>[3x]MSLNVQTVAVIGSGTMGAGIAEVAASHGHQVLLYDISAEALTRAIDGIHARLNSRVTRGKLTAETCERTLKRLI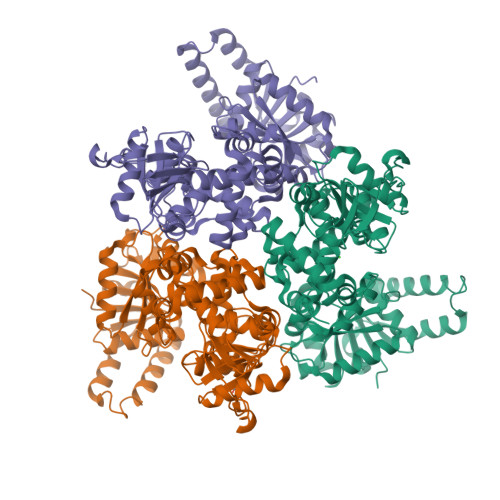PVTDIHALAAADLVIEAASERLEVKKALFAQLAEVCPPQTLLTTNTSSISITAIAAEIKNPERVAGLHFFNPAPVMKLVEVVSGLATAAEVVEQLCELTLSWGKQPVRCHSTPGFIVNRVARPYYSEAWRALEEQVAAPEVIDAALRDGAGFPMGPLELTDLIGQDVNFAVTCSVFNAFWQERRFLPSLVQQELVIGGRLGKKSGLGVYDWRAEREAVVGLEAVSDSFSPMKVEKKSDGVTEIDDVLLIETQGETAQALAIRLARPVVVIDKMAGKVVTIAAAAVNPDSATRKAIYYLQQQGKTVLQIADYPGMLIWRTVAMIINEALDALQKGVASEQDIDTAMRLGVNYPYGPLAWGAQLGWQRILRLLENLQHHYGEERYRPCSLLRQRALLESGYESEGHHHHHH> MEAFVPGVGPLLGAPAAPLAAVDVRCRHASVARRARVAVRMADDGFADLQPGDPGYKPKAKEMVKVSELGVSPFSDDANSVTRLGEGRLDEIAKDIMEGKKTGAEIKADLKKQAPAKPAAPAKKPEKKSGLASAKDAAGSAMGAVQRAVGSGKRGLDLLREDFLQTGPERAGVGRQD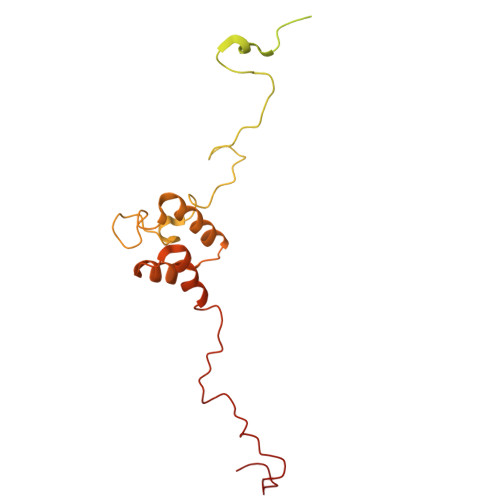KTVDAPPQFGEPGYVTPAYQRVKVSSLGISVFEDDANAVTKVGGIKAVMEVAEKVASGELKTEEFEEGLKAGLSLDLALEKMEEEAAAGDLLPDYLKPLPEDTPRKGMTWKNYVGR> MREVKEVDLRGLTVAEALLEVDQALEEARALGLSTLRLLHGKGTGALRQAIREALRRDKRVESFADAPPGEG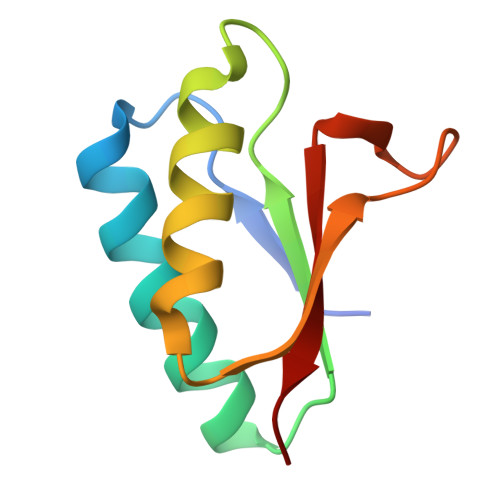GHGVTVVALRP> NNNGACUUA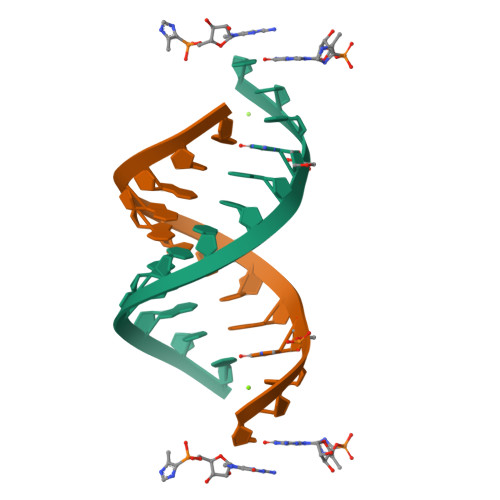AGUC> MKSVAILAALFGSATAFVPSQVSRTAASTSVKASLADMVGAEGPEPIPFAPSKTSKNFDPVGFAERSPEWLPWYREAELKHGRAAMLATVGFVVPEFIRVPGEQFSFEAIPKVIDAHDALPESMIQIFGWISFLEACTFPAMAGLGGKYDRKPGDFSFDPLGLYPTDPEKQKQMQLAELKNGRLAMIAIGGMVTGAAVTGHGFPYLP;> MKTAAIFALLAGSAAAFAPTTVSPRASTVAHMSSINEAFGISIETGNKCPPLGARILEDAQPSAIKWFQNAEIKHGRIAMVATIGYLVQKLGVHFPLYLGPSGSNCFHPESETAWLLSSSTGVTFSDIAKAAPLDAIQMVPVAGWMQIFFVAGWFESVAYYRQWVKNSPIPGDYGYDPLGFTKREGGWDSEELTSLRLKEIKNGRLAMMTIAAWVSDEMIPGALPVWHP;> MKSVLFLALAGSAAAFAPSTQSRSNTLLKADLSSLPGSTAPVGPFDPLNLADSGSEETLAWFRASELKHGRVAMLATTGYLVQGAGIHFPGMLSSDVSFESLSAMKPLEAWDAVPDAGKAQILGTIFIAEMITESKPVHYTKGGPMPTMVFPAIDFSGVDAATLKRKQDSELNNGRLAMIAIMSFISAANIPGSVPALTNNPAF;> MKLAILTTLLAGASAFTTPNARPAFATKLSMSEEAAAEEAPAADAPEEVVEPASPSYTCISKEAILSSPDTTEIGRVWDPLGLAEIGSAETLAWYRHSEVKHGRIAMAAFVGWWAVGAGLRFPGELSHGLEFSSIPSKGLEAWDAVPGWGKAQMLLFAGLIEFHDELFHTRRTEGGHYLRGGTPGKNMVPGLFDPFGFSKGKSEEELAKGRDREIKNGRLAMIGVAGLYCAATIPGSVPLQPPC;> MKIILSGLALLASSVAAFAPQSIISANANNKNANVVLEAAKDDLIAIAEKSNPVLKYYDPLQLGSTTIWGETNSATIGFLRQSEIKHGRIAMAAFVGYIVQANGIHFPWPMSFDGTPFPADAGSPPEQWDALSDAAKWQIILFIGFLEWFSEAAGKHYMRGGKPGAFPNFSDSDLIPHPVPLNLYDPFGFSKGKTEAQKADGLIKELNNGRLAMIGIMGFLAEQKVEGSVPLLKGVVPHYDGEVMAPFM;> MDNKIAGYNIIIHTIISSINMKFSLVVLSSLVVASSNGVTAFAPSSSTTSTSTTALSSSASKAELEAIAKKANPTLGYYDPLSLADKDFWGKGNDATIAFLRQSEIKHGRIAMFAFVGYIVQSNFVFPWAQTLAGAPHPSADLSPEAQWDAIPLGAKWQIFAVISALELWDECGGGGVLPHYTKGRKPGQYPPFTLFRDNVHFVLDLYDPFGFNKNMSEETKERRLVSELNNGR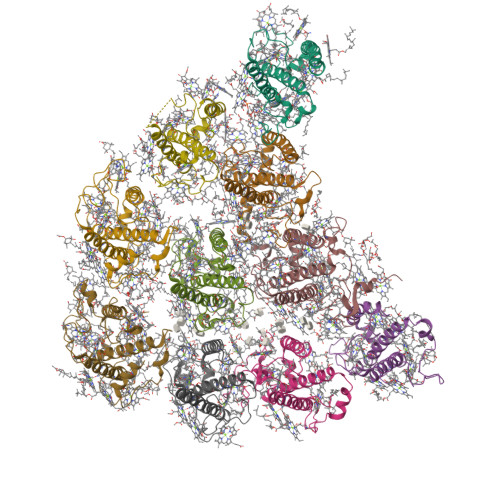LAMLGIFGFLCADTIPGSVPLLNDIAIPYSGQVMQPFEGQFSYFGSL;> MKIATLFLALASSAAAFAPSQQVRSMTNEKMKPRQARNNFALNMKVDEMPGATAPLGKFDPLNLATLGSESTLAWFRAAELKHSRVAMLATTGYLVQAAGIHFPGMLSSDVSFESLSAMKPLDAWDAVPEGGKNQIYFTIFLAEFITECKGTHYTKGGPLPTIVFPPIDFSTVNPEQLKTRQNRELNNGRLAMIAIMSFVAAANIPGSVPALAGNPMF;> MKLALLASLIASAAAFAPSSSTGAARASTALDAGKKSQALPFLPYPENLAGYVGDAGFDPFRFSDFAPMDFLREAEIKHGRICMLAWLGFVAVDLGARIYPLPEAYEGLTAVTAHDALVQQGAMSQIFLWCSVFEAISTVSVIQMLYEESGREPGYFGFDPLGFLNGKSEAEVNEMKLKEIKNGRLAMLAFSGVVTQAVLTQGPFPYV;> LLQGFSRWLVFFVSIRIIRHPCRPPYHETYSSSNTFLSIQYIEQSHSARQTSLSLLLITPLTLVLYLAIYTILKMFKTAAAITSLLAASASAFAPSSFNGRISTAVAAEKSQSLPFMNRPPLLDGSMAGDVGFDPLGLSNIDDVGIDLYWLREAEIKHCRVAMLAVVGILQVEIFGPAPGCEMATDKCQMDAFWQIWGAHPQYIAFGLIMIMMIEMISGIATTQGRESGERAPGDFGLDPLGYGKGDAAGYARLQAQEIANGRLAMFAAAGEIMQGCTTHQGALENLMTALRDNSF;> LRSIHHLIASHRRLFKFIRHYTINKMKSALIATALLAGSAAAFTSNAGSQSTSALKAMPERLWDSMVDKTERSKAVPFLPRAVNLDGSLPGDVGFDPFYLSSIPKDFSGFIQPPQWEEKGIPTLYWMREAELKHCRVAMLAWFGWLATDGAFGVTLRFPGEIYSVENIPTAYEAHNALVSQGSMGFLLLAVGFIEFCTGAVLVEVAKGASDREAGDFKLDPLSFLKGKSEEEIKRMKTREIANGRLAMLAFGGVATQTALEGGNHAFPYF> MSAEVIDRFFKSSGAGDIETAVECFADDGQWITPDGDGLGTVHTKDQIGDLITSMNAMREKMIASGVDGKFES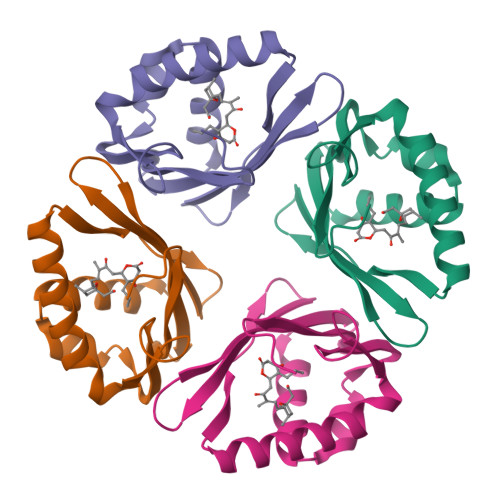PIMFGENMGLVRATVETDDGKVVNRGVDLFILSDGKIVLKDVYRKVKLAAALEHHHHHH>[2x]MMLKQ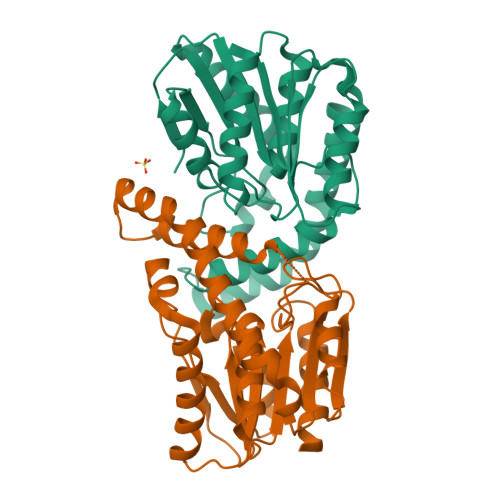PEPFFFEHGQHAVILLHAYAGSANDVRMLARALEREDYTVYGPQFSGHATDDPRDILAQTPAQWWQDTQQAISFMRQKGYTKISIFGLSLGGIFATAALERDPQLLGGGTFSSPLFAGNRSDVAEMFITLSHHQLAHSQFSIAEREQILMTLPELVQRQLQAVNTFTTTEVTSHLSAVTQPFFIGQGGQDELIDATVARQLRDQLPQVPVDFHWYADAGHVITVNSAHHQLEQDVLTYLKTIYK>MGKSLSHLPLHSSKEDAYDGVTSENMRNGLVNSEVHNEDGRNGDVSQFPYVEFTGRDSVTCPTCQGTGRIPRGQENQLVALIPYSDQRLRPRRTKLYVMAS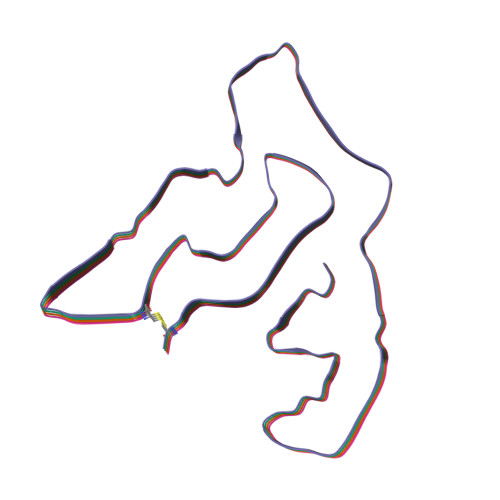VFVCLLLSGLAVFFLFPRSIDVKYIGVKSAYVSYDVQKRTIYLNITNTLNITNNNYYSVEVENITAQVQFSKTVIGKARLNNISIIGPLDMKQIDYTVPTVIAEEMSYMYDFCTLISIKVHNIVLMMQVTVTTTYFGHSEQISQERYQYVDCGRNTTYQLGQSEYLNVLQPQQ[4x]> MSGQFTGTGTGGDVFKVDLNEQFDRADMVWIGTASVLVWIMIPGVGLLYSGISRKKHALSLMWAALMAACVAAFQWFWWGYSLVFAHNGSVFLGTLQNFCLKDVLGAPSIVKTVPDILFCLYQGMFAAVTAILMAGAGCERARLGPMMVFLFIWLTVVYCPIAYWTWGGNGWLVSLGALDFAGGGPVHENSGFAALAYSLWLGKRHDPVAKGKVPKYKPHSVSSIVMGTIFLWFGWYGFNGGSTGNSSMRSWYACVNTNLAAATGGLTWMLVDWFRTGGK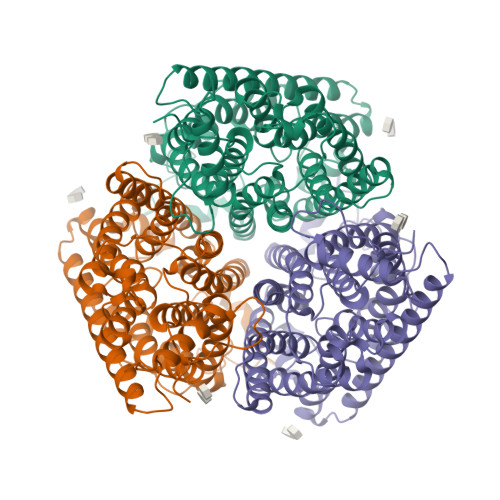WSTVGLCMGAIAGLVGITPAAGYVPVYTSVIFGIVPAIICNFAVDLKDLLQIDDGMDVWALHGVGGFVGNFMTGLFAADYVAMIDGTEIDGGWMNHHWKQLGYQLAGSCAVAAWSFTVTSIILLAMDRIPFLRIRLHEDEEMLGTDLAQIGEYAYYADDDPETNPYVLEPIDDTTISQPLPHIDGVADGSSNNDSGEAKNHHHHHH>MNINKHLMLLALLTNYSYANGNNITIPIEITQDAFHYISHKDLDKNIIDKYTIRQMNEYFNTQYYFQWSDDANQNDFYYVPNNTQTKNNILKLENDTIRYYKERSGYDKNYLPHTSNWVNSISENMNLKSFPNIPCDNHSCRGIVVNNAQVRSLPTSDAFYNNFTIPGEGYPFDYIQLSALWTGTPIMLIHMSTDKKWTLIKGQGTLGWVPTSSIANVDESFITQWKRYRLVTPTVRKQDLPIEKYDINNKILEAGSILPEHK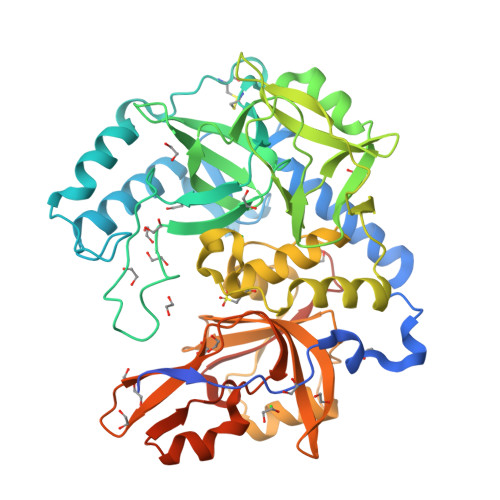GKLKIPVKDKNGTATLLTVNSKNLKFTTWPMTPSYKNFAHQINNYIGMPYGWGGMDFNNDCSGLLKRLFSTFGIWLPRSSFYQANYAGQIYSMYDQSEEQRKELLVEQEGSIQLIPFMTLVSFGNSKTSTSHIGLYMGTTEYNHNKVAIMFNAPWGVKLVNGNNEQGRALVGQTLITPIGIGDAFTEGLSNQDWALQSLWNAVGFNTTLLTETPKNKRLYQGIDNSYSIEKYLFEK[2x]> GHMLEDPKQLAVYEEFARNVPGFLPTNDLSQPTGFLAQPMKQAWATDDVAQIYDKCITELEQHLHAIPPTLAMNPQAQALRSLLEVVVLSRNSRDAIAALGLLQKAVEGLLDATSGADADLLLRYR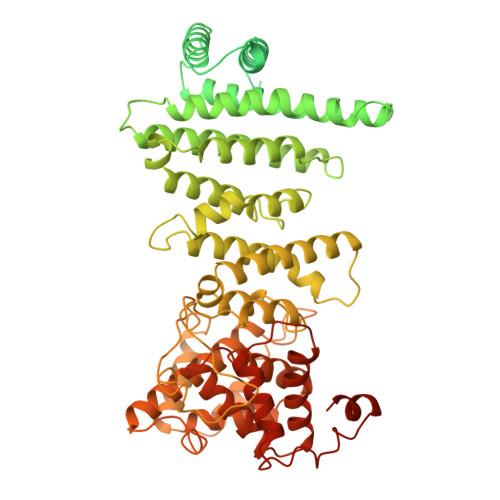ECHLLVLKALQDGRAYGSPWCNKQITRCLIECRDEYKYNVEAVELLIRNHLVNMQQYDLHLAQSMENGLNYMAVAFAMQLVKILLVDERSVAHVTEADLFHTIETLMRINAHSRGNAPEGLPQLMEVVRSNYEAMIDRAHGGPNFMMHSGISQASEYDDPPGLREKAEYLLREWVNLYHSAAAGRDSTKAFSAFVGQMHQQGILKTDDLITRFFRLCTEMCVEISYRAQAEQQHNPAANPTMIRAKCYHNLDAFVRLIALLVKHSGEATNTVTKINLLNKVLGIVVGVLLQDHDVRQSEFQQLPYHRIFIMLLLELNAPEHVLETINFQTLTAFCNTFHILRPTKAPGFVYAWLELISHRIFIARMLAHTPQQKGWPMYAQLLIDLFKYLAPFLRNVELTKPMQILYKGTLRVLLVLLHDFPEFLCDYHYGFCDVIPPNCIQLRNLILSAFPRNMRLPDPFTPNLKVDMLSEINIAPRILTNFTGVMPPQFKKDLDSYLKTRSPVTFLSDLRSNLQVSNEPGNRYNLQLINALVLYVGTQAIAHIHNKGSTPSMSTITHSAHMDIFQNLAVDLDTEGRYLFLNAIANQLRYPNSHTHYFSCTMLYLFAEANTEAIQEQITRVLLERLIVNRPHPWGLLITFIELIKNPAFKFWNHEFVHCAPEIEKLFQSVAQCCMGQKQAQQVME(1~{S})-~{N}-ethyl-1-(4-fluorophenyl)-1-[2-[4-[6-(1-methylpyrazol-4-yl)pyrrolo[2,1-f][1,2,4]triazin-4-yl]piperazin-1-yl]pyrimidin-5-yl]ethanamine 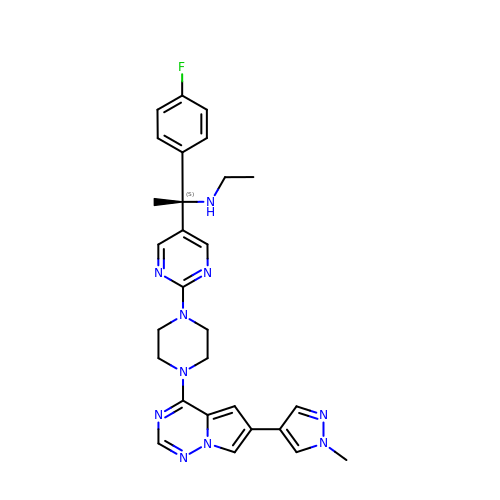| C28 H31 F N10 | XXXYMYPGZVMPNH-NDEPHWFRSA-N> GSMAEDADMRNELEEMQRRADQLAD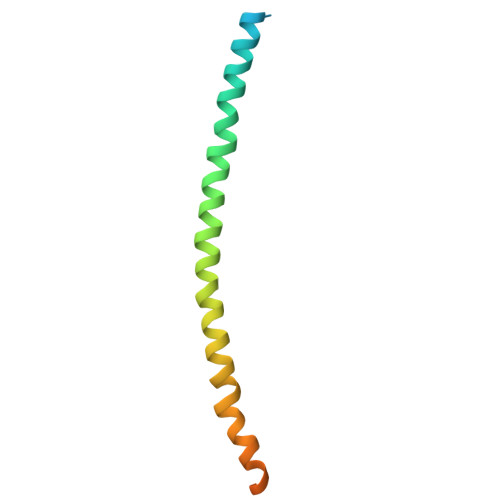ESLESTRRMLQLVEESKDAGIRTLVMLDEQGEQLERIEEGMDQINKDMKEAEKNLTDLGKFCGLCVCPCNKLKSSDA>[2x]MRSRRVDVMDVMNRLILAMDLMNRDDALRVTGEVREYIDTVKIGYPLVLSEGMDIIAEFRKRFGCRIIADFKVADIPETNEKICRATFKAGADAIIVHGFPGADSVRACLNVAEEMG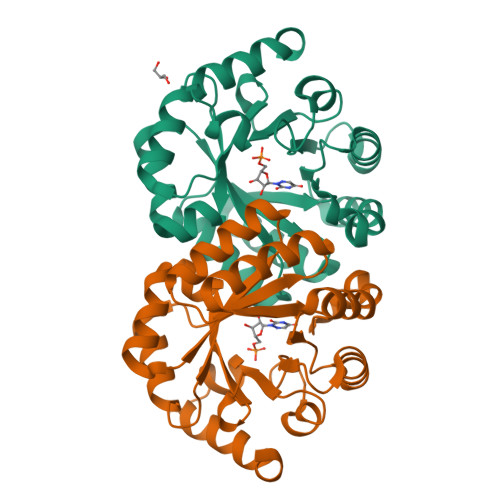REVFLSTEMSHPGAEMFIQGAADEIARMGVDLGVKNYVGPSTRPERLSRLREIIGQDSFLISPGVGAQGGDPGETLRFADAIIVGRSIYLADNPAAAAAGIIESIKDLLNP> RICPRIW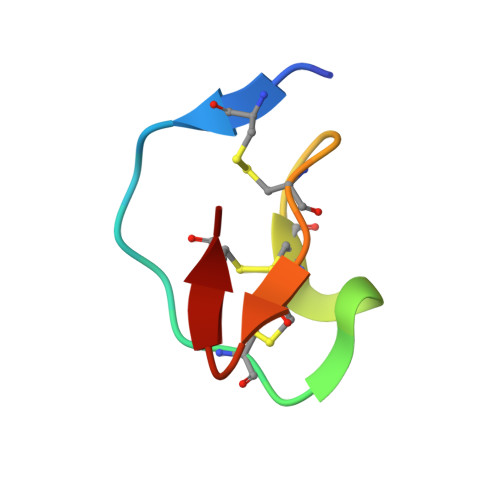MECKRDSDCMAECICVMGHCG>[2x]MAGKSAEEEHPIKAYGWAVKDRTTGILSPFKFSRRAT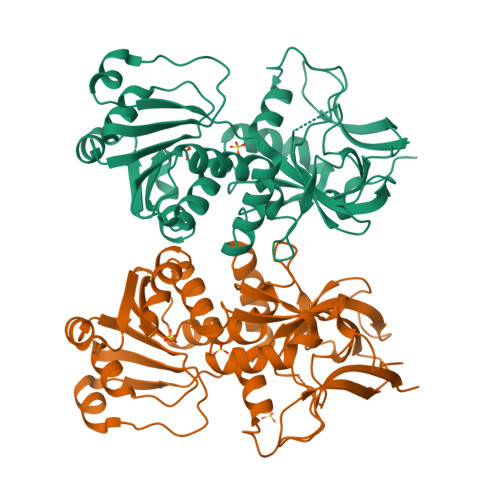GDDDVRIKILYCGICHTDLASIKNEYEFLSYPLVPGMEIVGIATEVGKDVTKVKVGEKVALSAYLGCCGKCYSCVNELENYCPEVIIGYGTPYHDGTICYGGLSNETVANQSFVLRFPERLSPAGGAPLLSAGITSFSAMRNSGIDKPGLHVGVVGLGGLGHLAVKFAKAFGLKVTVISTTPSKKDDAINGLGADGFLLSRDDEQMKAAIGTLDAIIDTLAVVHPIAPLLDLLRSQGKFLLLGAPSQSLELPPIPLLSGGKSIIGSAAGNVKQTQEMLDFAAEHDITANVEIIPIEYINTAMERLDKGDVRYRFVVDIENTLTPPSEL> MSVLDALWEDRDVRFDLSAQQMKTRPGEVLIDCLDSIEDTKGNNGDRGRLLVTNLRILWHSLALSRVNVSVGYNCILNITTRTANSKLRGQTEALYILTKCNSTRFEFIFTNLVPGSPRLFTSVMAVHRAYETSKMYRDFKLRSALIQNKQLRLLPQEHVYDKINGVWNLSSDQGNLGTFFITNVRIVWHANMNDSFNVSIPYLQIRSIKIRDSKFGLALVIESSQQSGGYVLGFKIDPVEKLQESVKEINSLHKVYSASPIFGVDYEMEEKPQPLEALTVEQIQDDVEIDSDGHTDAFVAYFADGNKQQDREPVFSEELGLAIEKLKDGFTLQGLWEVMS

The BBSome is a cargo adaptor that recognizes a diverse set of membrane-bound ciliary proteins. It binds with its cargo to the intraflagellar transport (IFT) complex, a large heterooligomeric protein complex that is transported along ciliary microtubules by the molecular motors dynein and kinesin. We recently reconstituted a heterologously expressed core complex of the human BBSome, comprising the subunits BBS1, 4, 5, 8, 9, and 18. Here we report the structure of the human BBSome core complex at an average resolution of 3.8 Å for BBS1, 4, 8, 9, and 18 and 4.3 Å for BBS5.

In addition, the resolution is limited in this region, indicating a high degree of conformational flexibility. After three-dimensional sorting we also resolved BBS5 at a resolution of 4.3 Å and combined its density with the reconstruction of the full data set to build an atomic model. BBS5 is composed of two PH domains that both interact with the β-propeller of BBS9. One of the PH domains also interacts with BBS8 and with an unstructured loop of BBS9. In the BBSome core structure, the PH domains are laterally rotated by 90° to each other. Like PH-GRAM and GLUE, BBS5 was shown to bind phosphoinositides, with the highest preference for phosphatidylinositol 3-phosphate (PI(3)P) and phosphatidic acid (PA), which was suggested to be crucial for ciliogenesis. Besides BBS1 that indirectly interacts with membranes via Arl6, BBS5 likely mediates the contact to membranes by direct interactions with phosphoinositides. Since the BBS5 and Arl6 binding sites are located on opposite sides of the core BBSome complex, a simultaneous membrane binding of both motifs would require a curved membrane surface, as it is present on the inner cilium wall, and/or conformational rearrangements of the complex. The observed dynamic properties of BBS5 (Figure 1—figure supplements 1 and 3) are probably the prerequisite for the subunit to be able to reorient and position one or both of its PH domains closer to the membrane, thereby enabling interaction with the membrane.>[2x]MAKKTKQRRPMGFPPGPPGLPFIGNIYSLAASSELPHVYMRKQSQVYGEIFSLDLGGISTVVLNGYDVVK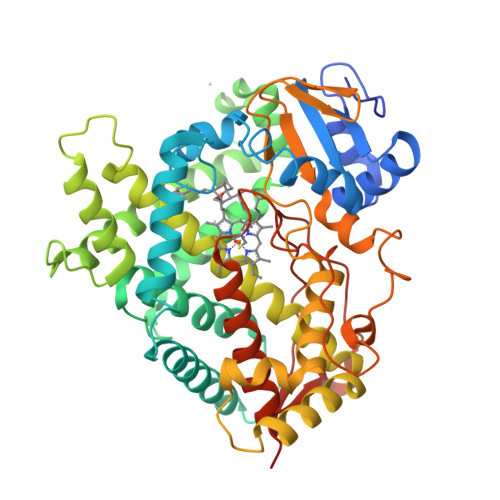ECLVHQSEIFADRPCLPLFMKMTKMGGLLNSRYGRGWVDHRRLAVNSFRYFGYGQKSFESKILEETKFFNDAIETYKGRPFDFKQLITNAVSNITNLIIFGERFTYEDTDFQHMIELFSENVELAASASVFLYNAFPWIGILPFGKHQQLFRNAAVVYDFLSRLIEKASVNRKPQLPQHFVDAYLDEMDQGKNDPSSTFSKENLIFSVGELIIAGTETTTNVLRWAILFMALYPNIQGQVQKEIDLIMGPNGKPSWDDKCKMPYTEAVLHEVLRFCNIVPLGIFHATSEDAVVRGYSIPKGTTVITNLYSVHFDEKYWRDPEVFHPERFLDSSGYFAKKEALVPFSLGRRHCLGEHLARMEMFLFFTALLQRFHLHFPHELVPDLKPRLGMTLQPQPYLICAERRHHHH> MFRILTINPGSTSTKLSIFEDERMVKMQNFSHSPDELGRFQKILDQLEFREKIARQFVEETGYSLSSFSAFVSRGGLLDPIPGGVYLVDGLMIKTLKSGKNGEHASNLGAIIAHRFSSETGVPAYVVDPVVVDEMEDVARVSGHPNYQRKSIFHALNQKTVAKEVARMMNKRY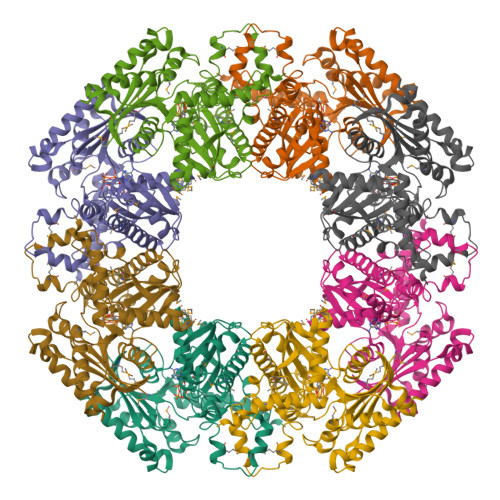EEMNLVVAHMGGGISIAAHRKGRVIDVNNALDGDGPFTPERSGTLPLTQLVDLCFSGKFTYEEMKKRIVGNGGLVAYLGTSDAREVVRRIKQGDEWAKRVYRAMAYQIAKWIGKMAAVLKGEVDFIVLTGGLAHEKEFLVPWITKRVSFIAPVLVFPGSNEEKALALSALRVLRGEEKPKNYSEESRRWRERYDSYLDGILRHHHHHH> GGGAEALELLEHCGV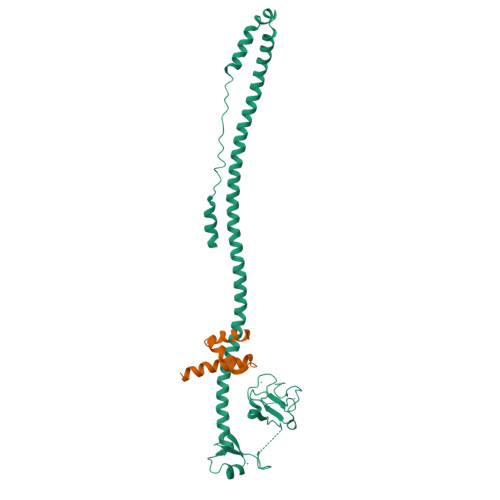CRERLRPEREPRLLPCLHSACSACLGPAAPAAANSSGDGGAAGDGTVVDCPVCKQQCFSKDIVENYFMRDSGSKAGERTVYCNVHKHEPLVLFCESCDTLTCRDCQLNAHKDHQYQFLEDAVRNQRKLLASLVKRLGDKHATLQKSTKEVRSSIRQVSDVQKRVQVDVKMAILQIMKELNKRGRVLVNDAQKVTEGQQERLERQHWTMTKIQKHQEHILRFASWALESDNNTALLLSKKLIYFQLHRALKMIVDPVEPHGEMKFQWDLNAWTKSAEAFGKIVAERPGTNSTGPAPMAPPRAPGPLSK;> LSELEDLKDAKLQTLKELFPQRSDNDLLKLIESTSTMDGAIAAALLMF> MRLTEEEVQALLEKADGWKLADERWIVKKYRFQDYLQGIEFVRRIAAISENANHHPFISID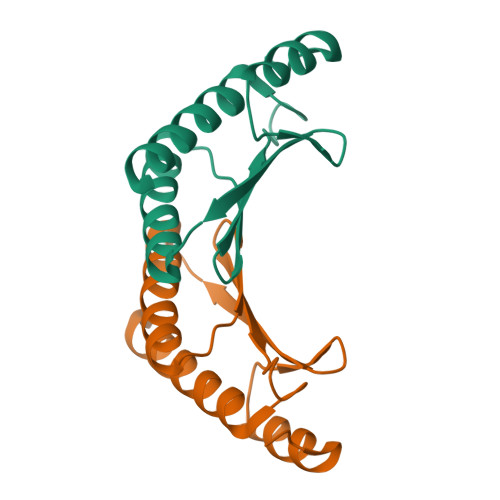YKLITVKLSSWRAKGLTKLDFDLAKQYDEVYNQMKQGEGE>[2x]WSHPQFEKGAETAVPNSEDVMKRAQGLFKPIPAKPPVMKDNPASPSRVELGRMLFFDPRLSASHLISCNTCHNVGLGGTDILE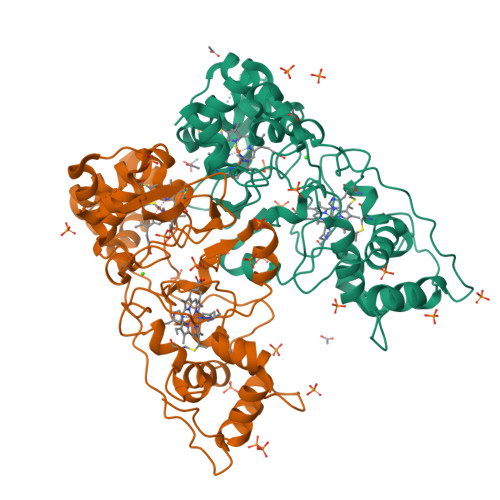TSIGHGWQKGPRNSPTVLNAVYNIAQFWDGRAEDLAAQAKGPVQASVEMNNKPENLVATLKSIPGYPPLFRKAFPGQGDPVTFDNVAKAIEVFEATLVTPDAPFDKYLKGNRKAISSTAEQGLALFLDKGCAACHSGVNMGGTGYFPFGVREDPGPVVRPVDDTGRYKVTSTAADKYVFRSPSLRNVAITMPYFHSGKVWKLKDAVKIMGSAQLGISITDADADKIVTFLNTLTGAQPKVMHPVLPPNSDDTPRPVSN>[2x]ASAWPEEKNYHQPAILNSSALRQIAEGTSISEMWQNDLQPLLIERYPGSPGSYAARQHIMQRIQRLQADWVLEIDTFLSQTPYGYRSFSNIISTLNPTAKRHLVLACHYDSKYFSHWNNRVFVGATDSAVPCAMMLELARALDKKLLSLKTVSDSKPDLSLQLIFFDGEEAFLHWSPQDSLYGSRHLAAKMASTPHPP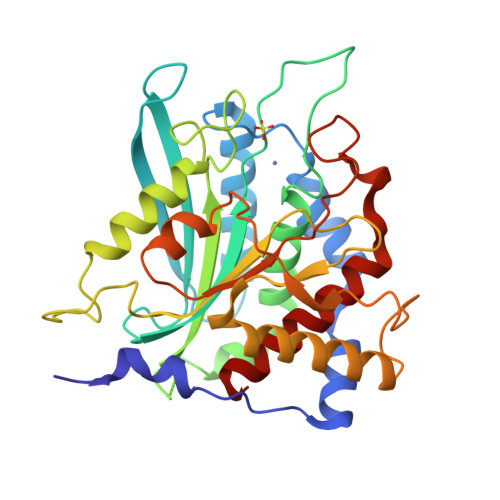GARGTSQLHGMDLLVLLQLIGAPNPTFPNFFPNSARWFERLQAIEHELHELGLLKDHSLEGRYFQNYSYGGVIQDDHIPFLRRGVPVLHLIPSPFPEVWHTMDDNEENLDESTIDNLNKILQVFVLEYLHL> GGSEGDTLGDMWKARLNSCTKEEFFAYRRAGVMETDREKARELLKRGETNMGLAVSRGTSKL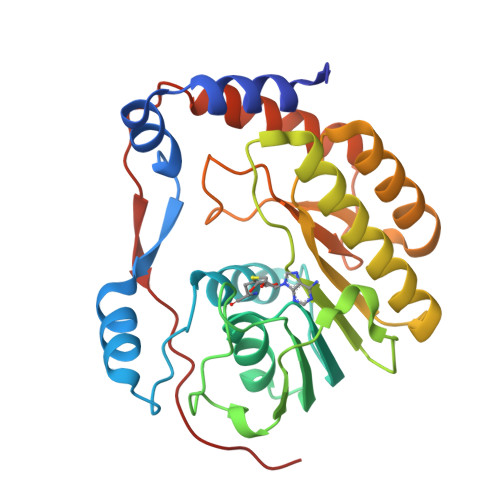AWMEERGYVTLKGEVVDLGCGRGGWSYYAASRPAVMSVRAYTIGGKGHESPRMVTSLGWNLIKFRAGMDVFSMEPHRADAILCDIGESNPDAVVEGERSRRVILLMEQWKNRNPTATCVFKVLAPYRPEVIEALHRFQLQWGGGLVRTPFSRNSTHEMYFSTAITGNIVNSVNIQSRKLLARFGDQRGPTRVPEIDLGVGTRCV>[2x]MKDCSNGCSAECTGEGGSKEVVGTFKAKDLIVTPATILKEKPDPNNLVFGTVFTDHMLTVEWSSEFGWEKPHIKPLQNLSLHPGSSALHYAVELFEGLKAFRGVDNKIRLFQPNLNMDRMYRSAVRATLPVFDKEELLECIQQLVKLDQEWVPYSTSASLYIRPTFIGTEPSLGVKKPTKALLFVLLSPVGPYFSSGTFNPVSLWANPKYV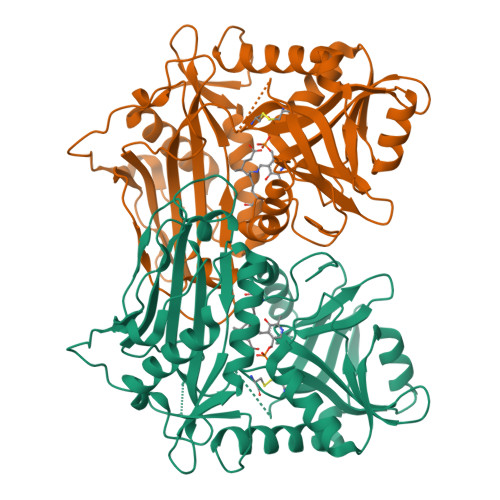RAWKGGTGDCKMGGNYGSSLFAQCEAVDNGCQQVLWLYGEDHQITEVGTMNLFLYWINEDGEEELATPPLDGIILPGVTRRCILDLAHQWGEFKVSERYLTMDDLTTALEGNRVREMFGSGTACVVCPVSDILYKGETIHIPTMENGPKLASRILSKLTDIQYGREERDWTIVLS> AAPGKPTIAWGNTKFAIVEVDQAATAYNNLVKVKNAADVSVSWNLWNGDTGTTAKVLLNGKEAWSGPSTGSSGTANFKVNKGGRYQMQVALCNADGCTASDATEIVVADTDGSHLAPLKEPLLEKNKPYKQNSGKVVGSYFVEWGVYGRNFTVDKIPAQNLTHLLYGFIPICGGNGINDSLKEIEGSFQALQRSCQGREDFKVSIHDPFAALQKAQKGVTAWDDPYKGNFGQLMALKQAHPDLKILPSIGGWTLSDPFFFMGDKVKRDRFVGSVKEFLQTWKFFDGVDIAWEFPGGKGANPNLGSPQDGETYVLLMKELRAMLDQLSVETGRKYELTSAISAGKDKIDKVAYNVAQNSMDHIFLMSYDFYGAFDLKNLGHQTALNAPAWKPDTAYTTVNGVNALLAQGVKPGKIVVGTAMYGRGWTGVNGYQNNIPFTGTATGPVKGT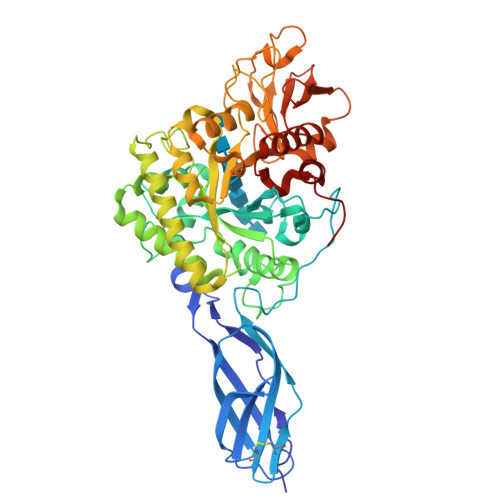WENGIVDYRQIAGQFMSGEWQYTYDATAEAPYVFKPSTGDLITFDDARSVQAKGKYVLDKQLGGLFSWEIDADNGDILNSMNASLGNSAGVQ> MEKRQARNSGVRKEDVGWWDPNPAADGNMHLGLNFDRLKYWLTAGAK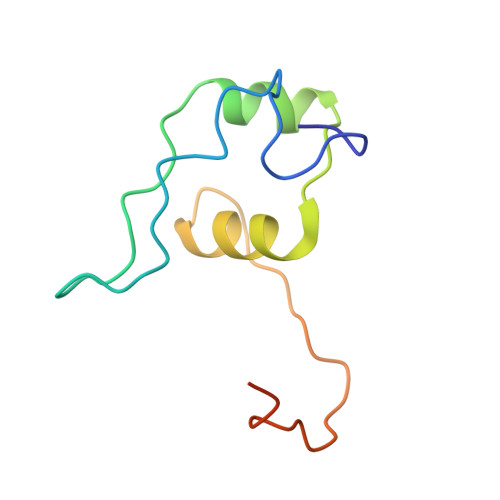PTDKVAELLGHAGVLPKVPQPPHYNPRDPKDDTKWRPNEDK>MGAIESRKLLASETPVGQFIPYSHHVTDTIISTKNAEYLSVWKIDGRSHQSASEADVFQWIRELNNTLRGISSANLSLWTHIVRRRVYEYPDAEFDNVFCRQLDEKYRESFTGYNLMVNDLYLTVVYRPVSDKVLSFFAKRERETPDQKKHRQESCIKALEDINRTLGQSFKRYGAELLSVYEKGGHAFSAPLEFLARLVNGEHIPMPICRDRFSDYMAVNRPMFSKWGEVGELRSLTGLRRFGMLEIREYDDATEPGQLNVLLESDYEFVLTHSFSVLSRPAAKEYLQRHQKNLIDARDVATDQIEEIDEALNQLISGHFVMGEHHCTLTVYGETVQQVRDNLAHASAAMLDVAVLPKPVDLALEAGYWAQLPANWQWRPRPAPITSLNFLSFSPFHNFMSGKPTGNPWGPAVTILKTVSGTPLYFNFHASKEEEDATDKRLLGNTMLIGQSSSGKTVLLGFLLAQAQKFKPTIVAFDKDRGMEISIRAMGGRYLPLKTGEPSGFNPFQLPPTHANLIFLKQFVKKLAAAGGEVTHRDEEEIDQAITAMMSDSIDKSLRRLSLLLQFLPNPRSDDMDARPTVHARLVKWCEGGDYGWLFDNPTDALDLSTHQIYGFDITEFLDNPEARTPVMMYLLYRTESMIDGRRFMYVFDEFWKPLQDEYFEDLAKNKQKTIRKQNGIFVFATQEPSDALESNIAKTLIQQCATYIFLANPKADYEDYTQGFKLTDSEFELVRGLGEFSRRFLIKQGDQSALAEMNLGKFRTIVDGETVERDFDDELLVLSGTPDNAEIAESIIAEVGDDPAVWLPIFLDRVKAERSDVGSGSGSAVDMFIKIGDVKGESKDKTHAEEIDVLAWSWGMSQSGSMHMGGGGGAGKVNVQDLSFTKYIDKSTPNLMMACSSGKHYPQAKLTIRKAGGENQVEYLIITLKEVLVSSVSTGGSGGEDRLTENVTLNFAQVQVDYQPQKADGAKDG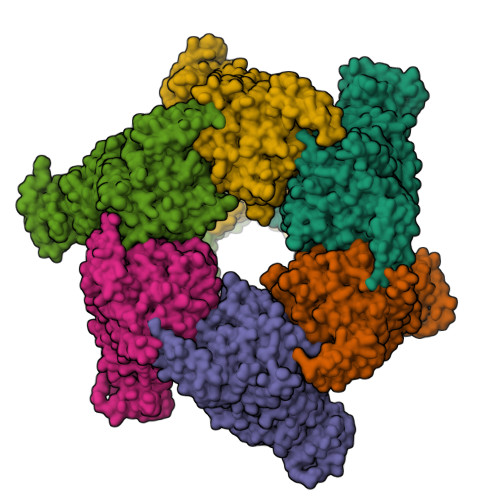GPVKYGWNIRQNVQA[6x]> MVSQPIKLLVGLANPGPEYAKTRHNAGAWVVEELARIHNVTLKNEPKFFGLTGRLLINSQELRVLIPTTFMNLSGKAIAAL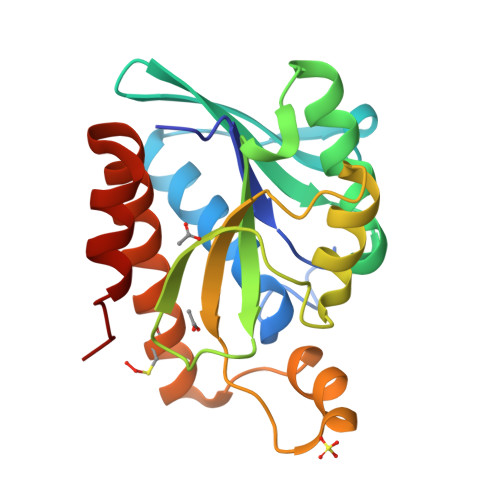ANFYQIKPEEIMVAHDELDLPPGVAKFKQGGGHGGHNGLKDTISKLGNNKEFYRLRLGIGHPGHKDKVAGYVLGKAPAKEQECLDAAVDESVRCLEILMKDGLTKAQNRLHTFKAE> MSKEIPTPYMWSYQPQMGLAAGAAQDYSTRMNWLSAGPAMISRVNDIRAHRNQILLEQSALTATPRNHLNPRNWPAALVYQEIPQPTTVLLPRDAQAEVQLTNSGVQLAGGATLCRHRPAQGIKRLVIRGRGTQLND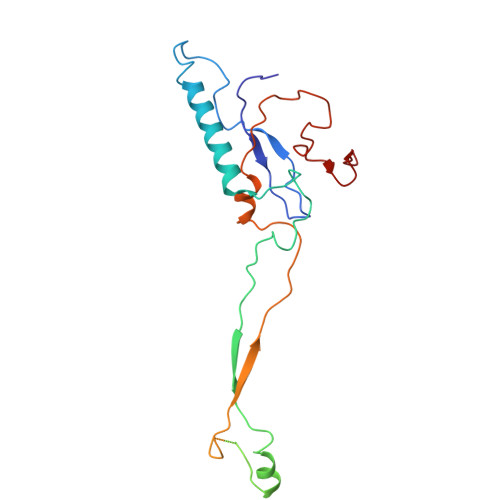EVVSSSLGLRPDGVFQLAGSGRSSFTPRQAVLTLESSSSQPRSGGIGTLQFVEEFTPSVYFNPFSGSPGHYPDEFIPNFDAISESVDGYD>[3x]GPGSKPFTLPILTLGELTNSRFPLPIDVLYTNPNESAIVQCQNGRCTLD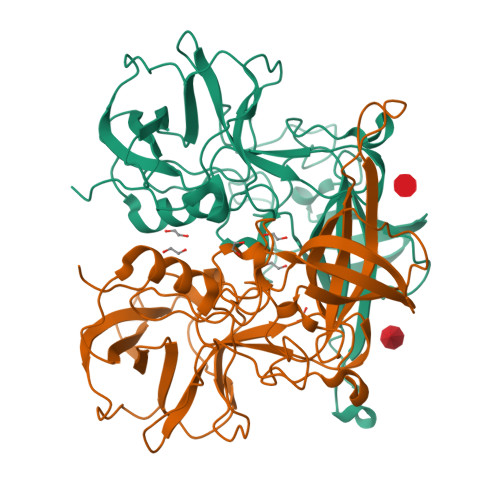GELQGTTQLLPTGICAFRGKVTQQVQDEHRGTHWNMTVTNLNGTPFDPTEDVPAPLGTPDFSGQIYGVISQRNTNTVPGEGNLPANRAHEAVIATYSPKFTPKLGNIQFSTWETQDVSSGQPTKFTPVGLASVDANSHFDQWTLPSYSGALTLNMNLAPSVAPVFPGECLLFFRSFIPLKGGYGNPAIDCLMPQEWVQHLYQESAPSLSDVALVRYVNPETGRTLFEAKLHRNGFLTVARNSAGPVVAPTNGYFRFDSWVNQFYTLAPM> MSQSVSERTRIKSDRYESGVIPYAKMGYWDAAYTVKDTDVLALFRITPQPGVDPVEAAAAVAGESSTATWTVVWTDLLTACERYRAKAYRVDPVPNSTDVYFAFIAYECDLFEEASLANLTASIIGNVFGFKAISALRLEDMRIPHSYLXTFQGPATGIIVERERLNKYGTPLLGATVKPKLGLSGKNYGR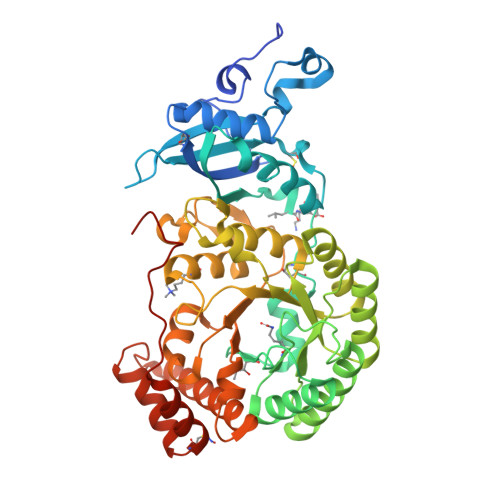VVYEGLKGGLDFLKDDENINSQPFMRWRERFLNCLEGINRASAATGEVKGSYLNVTAATMEEVYKRAEYAKAIGSIVVMIDLVMGYTAIQSIAYWARENDMLLHLHRAGNSTYARQKNHGINFRVICKWMRMSGVDHIHAGTVVGKLEGDPLMIKGFYDILRLTELEVNLPFGIFFEMDWASLRRCMPVASGGIHCGQMHQLIHYLGDDVVLQFGGGTIGHPDGIQAGATANRVALEAMVLARNEGADYFNNQVGPQILRDAAKTCGPLQTALDLWKDISFNYTSTDTADFSETATANR>[2x]GQYDDHPPVFQKKFYIGGVSEDARMFASVLRVKATDRDTGNYSAMAYRLIIPPIKEGKEGFVVETYTGLIKTAMLFHNMRRSYFKFQVIATDDYGKGLSGKADVLVSVVNQLDMQVIVSNVPPTLVEKKIEDLTEILDRYVQEQIPGAKVVVESIGARRHGDAYSLEDYSKCDLTVYAIDPQTNRAIDRNELFKFLDGKLLDINKDFQPYYGEGGRILEIRTPEAVTSIKKRGESLGYTEGALLALAFIIILCCIPAILVVLVSYRQFKVRQAECTKTARIQSAMPAAKPAAPVPAAPAPPPPPPPPPPGAHLYEELGESAMHKYETALFESRLVPR;>GSGGRATMVKLLPAQEAAKIYHTNYV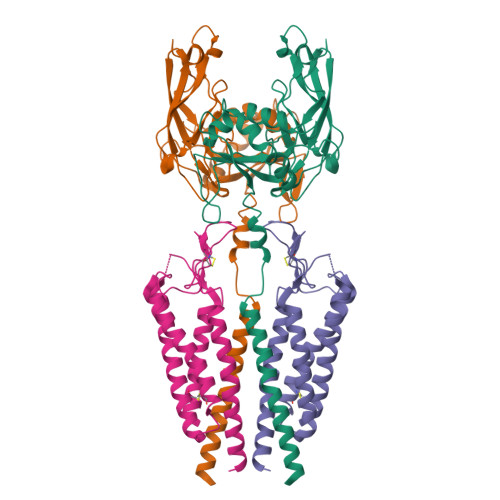RNSRAVGVMWGTLTICFSVLVMALFIQPYWIGDSVSTPQAGYFGLFSYCVGNVLSSELICKGGPLDFSSIPSRAFKTAMFFVALAMFLIIGSIICFSLFFVCNTATVYKICAWMQLAAATGLMIGCLVYPDGWDSSEVRRMCGEQTGKYTLGHCTIRWAFMLAILSIGDALILSFLAFVLGYRQDKLLPDDYKADGNEEVFE[2x]2,4-bis(aziridin-1-yl)-6-(1-phenylpyrrol-2-yl)-1,3,5-triazine | C17 H16 N6 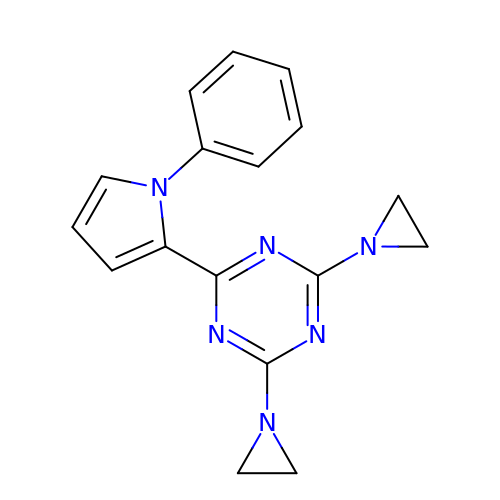| DAZONCQAIYYVKR-UHFFFAOYSA-N>HHHHHHSSGLVPRGSHMFRSSLTHLQAASRVFIVGGHITPFVGKGSPLFIDKKHPDFGKKKNMTLEEILATTVQGTMEHSGLSGREGIVDQVVVGNFLGELFSSQGHLGPAAIGSLTYGQAGSKNPLMYKPAMRVEGAAASGGLAVISAMNALKSGSADITLAVGVEVQTTASARVGGDYLARAADYQRQRQLDDFTFPCLFAKRMKYIAEHNHFTMEDTARVAAKAYANGNKNPLAHMHTRKLTFEQCNGEDPSNVKFLGNETYKEYLRMTDCSQVSDGGAGVVLANEEGLRKMGLSPNDSRLVEIKSIACAVSNLYEDPDDACCMFTSRQAAQKAL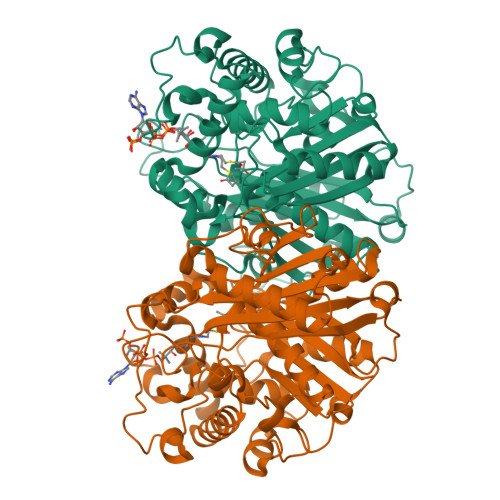SMANIKPSDLNVAEVHDCFTIAEMLMYEALGIAEYGHAKDLIRNGDTTLEGRIPVNTGGGLLSFGHPVGATGIKQIMEVYRQMKGQCEAYQMKKIPALGATLNMGGDDKTAVSAVLQNI[4x]>[2x]VRLPGLAAMRQGTRLFTPEQGEDLREALRRRRGSFQTTCEVTSETTFAAARRLREKASALAALNF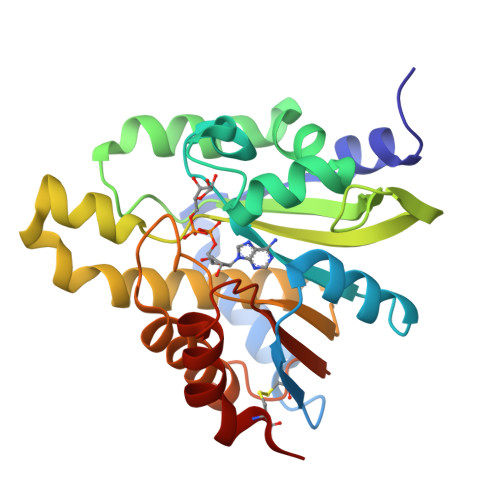ASAKNPGGGFLGGAQAQEEDLCRGSGLYFSLTSPQAEPYYAVNRQSHSALYTDHLIYSPQVPIFRDDAGQLLPAPVPVNIITAPAPNAGAVAQSRPEQLPQVLPTLRERARRVLGVAAWMEQTHLVLGAWGCGVFRNDPAGVARTFRELLEGEAQGAFEHVTFAVLDNHPQHPTLGAFRRELESLCLP>[2x]QGNDTSEVMLLDTGWEFSQSGTEKWMPATVPGTVHQDLISHELLPNPFYGMNEKKIQWVENEDWEYRTSFIVSEEQLNRDGIQLIFEGLDTYADVYLNGSLLLKADNMFVGYTLPVKSVLRKGENHLYIYFHSPIRQTLPQYASNGFNYPADNDHHEKHLSVFSRKAPYSYGWDWGIRMVTSGVWRPVTLRFYDIATISDYYVRQLSLTDENARLSNELIVNQIVPQKIPAEVRVNVSLNGTTVTEVKQQVTLQPGINHITLPAEVTNPVRWMPNGWGTPTLYDFSAQIACGDRIVAEQSHRIGLRTIRVVNEKDKDGESFYFEVNGIPMFAKGANYIPQDALLPNVTTERYQTLFRD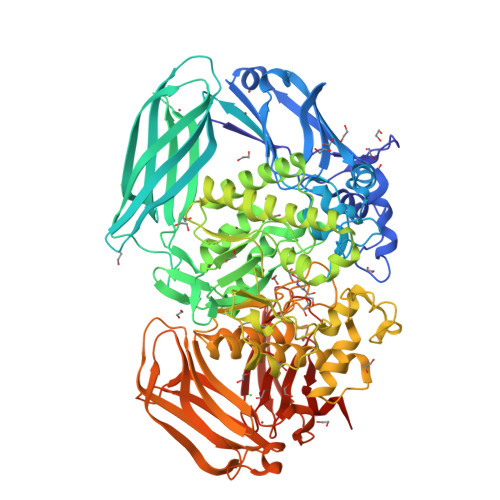MKEANMNMVRIWGGGTYENNLFYDLADENGILVWQDFMFACTPYPSDPTFLKRVEAEAVYNIRRLRNHASLAMWCGNNEILEALKYWGFEKKFTPEVYQGLMHGYDKLFRELLPSTVKEFDSDRFYVHSSPYLANWGRPESWGTGDSHNWGVWYGKKPFESLDTDLPRFMSEFGFQSFPEMKTIAAFAAPEDYQIESEVMNAHQKSSIGNSLIRTYMERDYIIPESFEDFVYVGLVLQGQGMRHGLEAHRRNRPYCMGTLYAQLNDSWPVVSWSSIDYYGNWKALHYQAKRAFAPVLINPIQQNDSLSVYLISDRLDTMEQMTLEMKVVDFDGKTLGKKIQVHSLEVPANTSKCVYRAKLDGWLTPEDCRRSFLKLILKDKSGHQVAESVHFFRKTKDLQLPPTSVSYQMKQTDGKCELTLFSSMLAKDIFIETPLQGARYSDNFFDLLPGERKKVIITSPRIKKGEELPVNIKHIRETYKEHHHHHH> MSLSEGTFEVGKNTFLLNGE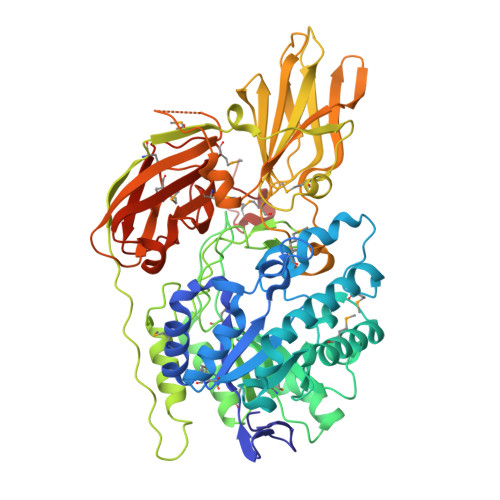PFVVKAAEIHYPRIPKEYWEHRIKMCKALGMNTICLYVFWNFHEPEEGRYDFAGQKDIAAFCRLAQENGMYVIVRPGPYVCAEWEMGGLPWWLLKKKDIKLREQDPYYMERVKLFLNEVGKQLADLQISKGGNIIMVQVENEYGAFGIDKPYISEIRDMVKQAGFTGVPLFQCDWNSNFENNALDDLLWTINFGTGANIDEQFKRLKELRPDTPLMCSEFWSGWFDHWGAKHETRSAEELVKGMKEMLDRNISFSLYMTHGGTSFGHWGGANFPNFSPTCTSYDYDAPINESGKVTPKYLEVRNLLGNYLPEGETLPEIPDSIPTIAIPTIKMTEMAVLFDNLPHPKESEDIRTMEAFDQGWGSILYRTSLSASDKEQTLLITEAHDWAQVFLNGKKLATLSRLKGEGVVKLPPLKEGDRLDILVEAMGRMNFGKGIYDWKGITEKVELQSDKGVELVKDWQVYTIPVDYSFARDKQYKQQENAENQPAYYRSTFNLNELGDTFLNMMNWSKGMVWVNGHAIGRYWEIGPQQTLYVPGCWLKKGENEIIILDMAGPSKAETEGLRQPILDVQRGNGAYAHRKMGEGHHHHHH D-valyl-N-[(2S,3S)-7-amino-1-chloro-2-hydroxyheptan-3-yl]-L-leucinamide 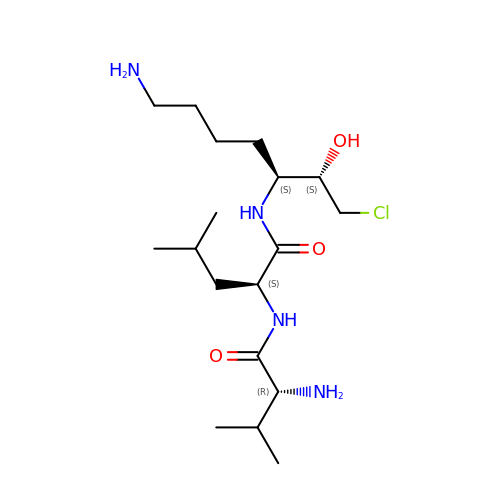| C18 H37 Cl N4 O3 | NJRUTHUXGPMPJA-CAOSSQGBSA-N>FAIQIVTVRSGDSVYSLASKYGSTPDEIVKDNGLNPAETLVVGQALIVNTKGNNYYVQPGDSLYRISQTYNVPLASLAKVNNLSLKSILHVGQQLYVPKGTKRSVESIAYLQPSTIPIKESLVNATRAINPFLTYLAYFSFEAKRDGTLKEPTETAKIANIATQGQTIPMLVITNIENGNFSADLTSVILRDATIQNKFITNILQTAEKYGMRDIHFDFESVAPEDREAYNRFLRNVKIRLPSGYTLSTTLVPKTSSNQKGKFFEAHDYKAQGQIVDFVVIM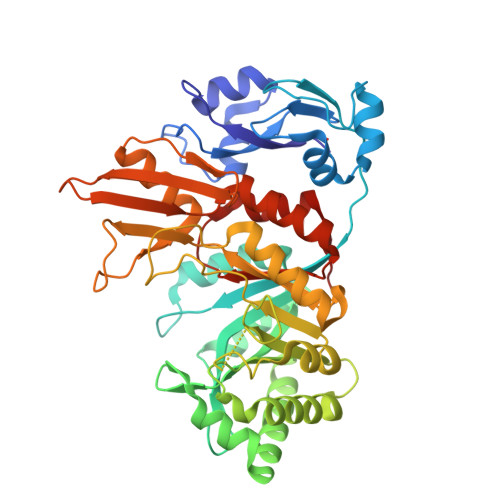TYDWGWQGGPPMAISPIGPVKEVLQYAKSQMPPQKIMMGQNLYGFDWKLPFKQGNPPAKAVSSVAAVALARKYNVPIRYDFTAQAPHFNYFDENGVQHEVWFEDARSIQSKFNLMKEQGIGGISYWKIGLPFPQNWRLLVENFTITKKGEN[3x]Fosfomycin-resistance proteins (FosAs) are dimeric metal-dependent glutathione transferases that conjugate the antibiotic fosfomycin (Fos) to the tripeptide glutathione (γ-Glu-Cys-Gly, GSH), rendering it inactive. FosA enzymes are manganese (Mn+2)- and potassium (K+)-dependent glutathione transferases that conjugate GSH to carbon 1 (C1) of Fos, leading to the opening of the epoxide ring of Fos. The catalytically active form of the FosA enzyme is a homodimer, whose tertiary structure complies with the fold of members of the VOC superfamily of enzymes. Members of the VOC family share a common fold composed of two βαβββ units that form an incompletely closed β-sheet barrel.

The crystal structure of the dimeric FosAKP was determined via X-ray crystallography at 1.48 Å resolution. The three-dimensional structure of FosAKP is folded into a dimer, providing an active site per monomer. Both subunits are composed of two tandem βαβββ motifs that follow a 3D-domain swapping during homodimer formation. Consequently, each active site was formed by residues originating from both subunits. A Fos molecule was found bound in the actives site of the first molecule of the dimer. In the active site of the second molecule, a tartrate molecule was bound, which originated from the crystallization buffer. Important residues that play crucial role in Fos binding include Ser97, Lys93, His67, Tyr65, Arg122, Glu113, and Tyr103. Mn2+ binding was coordinated by two His residues (His7 and His67) and Glu113. However, two additional residues (Tyr131 from molecule A and Tyr39 from molecule B of the dimer) appeared to contribute significantly to Tar binding. In particular, the C-terminal part of the Tar-bound subunit appears to be less solvent accessible, suggesting the formation of a more compact complex.

>[2x]MLSGLNHLTLAVSQLAPSVAFYQQLLGMTLHARWDSGAYLSCGDLWLCLSLDPQRRVTPPEESDYTHYAFSISEADFASFAARLEAAGVAVWKLNRSEGASHYFLDPDGHKLELHVGSLAQRLAACREQPYKGMVFFEQKGHHHHHH> MTQCYAEITGWGKCLPPATLSNHDLSTFLDTSDEWIQSRTGIEQRRISHVNTSDLATVAAQHAIACAGVSVEEIDLIIVATCSPDSLIPNIASRVQQNLGIPSAAAFDLNAACTGFLYGLETATRLMQASHYRHALVIGAERLSFYLDWTKRDTAVLFGDGAGAVVLSKTEQKVGLQDAQIGCDAQGRDILAVPKFGTAMDRFDADNGYWAFDFVGKEIFKRAVRGMGAAAQQVLARSGLSTEEIDVVIPHQANIRIIQTLCDLAGIAQDKAFVNIHRYGNTSAATVPIALCEALEQGKIKPHDDLLVAAFGAGLTWGAGHIRWGERITPLGKSDAQLPSCDHTALDLLSKAIEHCKRHQS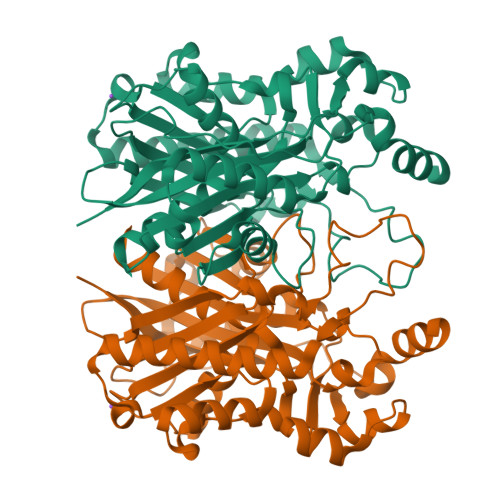E The core of the glideosome consists of an atypical class XIV myosin A (PfMyoA) and a divergent actin (PfAct1). PfMyoA is a short myosin with a conserved globular motor domain and a lever arm that binds two light chains: an essential light chain (PfELC) and myosin tail interacting protein (MTIP). PfMyoA is a critical molecule in the parasite life-cycle because it powers the fast motility (~2 µm.s−1) required during motile sporozoite stages, and is essential for providing the force (up to 40 pN) needed for non-motile merozoites to invade erythrocytes. Here, we present the X-ray structures of full-length (FL) PfMyoA complexed to PfELC and MTIP in two states of the motor cycle.

We determined the crystal structures of FL PfMyoA with two light chains bound (PfMyoA/PfELC/MTIP-Δn) in the post-rigor (PfMyoA•FL-PR) and in the pre-powerstroke (PfMyoA•FL-PPS) states at 2.5 Å and 3.9 Å resolution, respectively. The converter orientation is the same in both the motor domain (PfMyoA•MD-PR) and the FL (PfMyoA•FL-PR) post-rigor structures. Major differences are located at the ELC/converter interface when the PR and the PPS are compared, predominantly due to a sharp kink in the pliant region observed in the PR structures that promotes contacts between the ELC and the motor domain. SAXS experiments demonstrate that this ‘folded-back’ position of the lever arm is not primarily populated in solution and is selected by crystal contacts. In solution, the lever arm adopts an extended conformation as seen in other myosins. In PfMyoA, W777 is sandwiched between the α5*, α5’* and α6 helices, thus interacting with the hydrophobic core of the PfELC C-lobe. These interactions between W777 and the α5* and α5’* helices are not present in the folded-back PR structure that displays a much larger kink at the pliant region and thus moves W777 away. The absence of electron density for the two helical turns of α5* and α5’* in this crystal structure indicates that lack of stabilization by the converter and the W777 side chain affects the fold of these atypical PfELC structural elements. For all three structures, the electron density was well-defined for the motor domain and the lever arm, in particular for the interfaces between the HC and the PfELC and the interface between the two light chains.

> MAVTNEEIKTASKIVRRVSNVEAFDKSGSVFKGYQIWTDISPTIENDPNIMFVKCVVQQGSKKEKLTVVQIDPPGTGTPYDIDPTHAWNCNSQVDPMSFGDIGLLNHTNIPCVLDFLKHRYLKNQIYTTAVPLIVAINPYKDLGNTTNEWIRRYRDTADHTKLPPHVFTCAREALSNLHGVNKSQTIIVSGESGAGKTEATKQIMRYFASSKSGNMDLRIQTAIMAANPVLEAFGNAKTIRNNNSSRFGRFMQLVISHEGGIRYGSVVAFLLEKSRIITQDDNERSYHIFYQFLKGANSTMKSKFGLKGVTEYKLLNPNSTEVSGVDDVKDFEEVIESLKNMELSESDIEVIFSIVAGILTLGNVRLIEKQEAGLSDAAAIMDEDMGVFNKACELMYLDPELIKREILIKVTVAGGTKIEGRWNKNDAEVLKSSLCKAMYEKLFLWIIRHLNSRIEPEGGFKTFMGMLDIFGFEVFKNNSLEQLFINITNEMLQKNFVDIVFERESKLYKDEGISTAELKYTSNKEVINVLCEKGKSVLSYLEDQCLAPGGTDEKFVSSCATNLKENNKFTPAKVASNKNFIIQHTIGPIQYCAESFLLKNKDVLRGDLVEVIKDSPNPIVQQLFEGQVIEKGKIAKGSLIGSQFLNQLTSLMNLINSTEPHFIRCIKPNENKKPLEWCEPKILIQLHALSILEALVLRQLGYSYRRTFEEFLYQYKFVDIAAAEDSSVENQNKCVNILKLSGLSESMYKIGKSMVFLKQEGAKILTKIQREKLVEWENCVSVIEAAILKHKYKQKVNKNIPSLLRVQAHIRKKMVAQ;> MKQECNVCYFNLPDPESTLGPYDNELNYFTWGPGFEYEPEPQRKPLSIEESFENSEESEESVADIQQLEEKVDESDVRIYFNEKSSGGKISIDNASYNARKLGLAPSSIDEKKIKELYGDNLTYEQYLEYLSICVHDKDNVEELIKMFAHFDNNCTGYLTKSQMKNILTTWGDALTDQEAIDALNAFSSEDNIDYKLFCEDILQ;> MASDMEEKFREAFILFSSCSDHIEMYKFFELMNSFGIILTNDEKAALPNDINMDYWLNFAKKHYNYEQPFKHINNVNEQNTNVQIKIDNFLGIMKALDTRLTESDLNILLQITNPENKSTLNLKTVSQKLTESI>LQKAVEITYNGKTLRGLLHLPDDVKGKVPLVILFHGFTGNKVESHFIFVKLSRALEKVGIGSVRFDFYGSGESDGDFSELTFSSELEDARQILKFVKEQPTTDPERIGLLGLSLGGAIAGIVAREYKDEIKALVLWAPAFNLPELILNESVKQYGAILEQLGFVDIGGHKLSKDFVEDISKLNIFELSKGYDKKVLIVHGTNDEAVEYKVSDRILK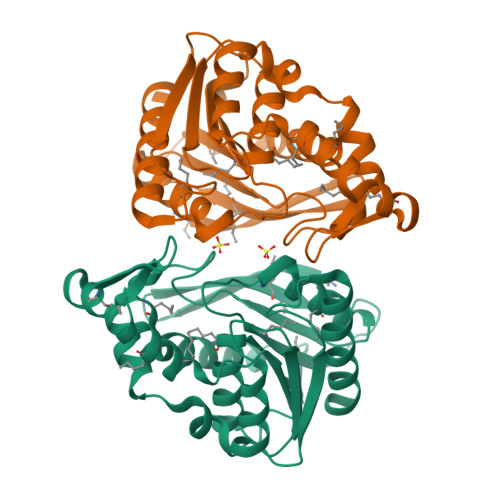EVYGDNATRVTIENADHTFKSLEWEKKAIEESVEFFKKELLKGGSHHHHHH[6x]>VRSSSRTPSDMPVAHVVANPQAEGQLQWLNRRANALLANGVELRDNQLVVPSEGLYLIYSQVLFSGQGCP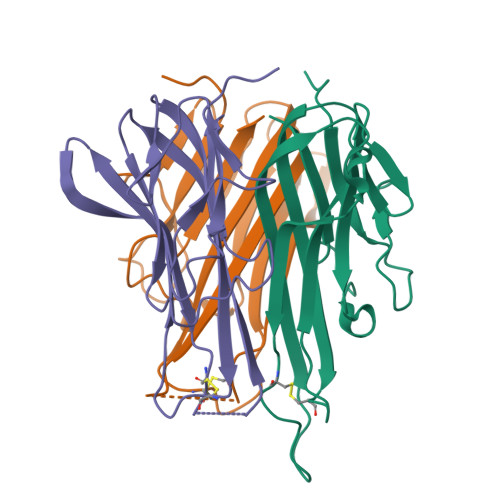STHVLLTHTISRISTTHNQPVNLLSAIRSPCQRETPEGAEANPWYEPIYLGGVFQLEPGDRLSAEINRPDYLDFAESGQVYFGIIAL[3x]>MSQFDILCKTPPKVLVRQFVERFERPSGEKIASCAAELTYLCWMITHNGTAIKRATFMSYNTIISNSLSFDIVNKSLQFKYKTQKATILEASLKKLIPAWEFTIIPYNGQKHQSDITDIVSSLQLQFESSEEADKGNSHSKKMLKALLSEGESIWEITEKILNSFEYTSRFTKTKTLYQFLFLATFINCGRFSDIKNVDPKSFKLVQNKYLGVIIQCLVTETKTSVSRHIYFFSARGRIDPLVYLDEFLRNSEPVLKRVNRTGNSSSNKQEYQLLKDNLVRSYNKALKKNAPYPIFAIKNGPKSHIGRHLMTSFLSMKGLTELTNVVGNWSDKRASAVARTTYTHQITAIPDHYFALVSRYYAYDPISKE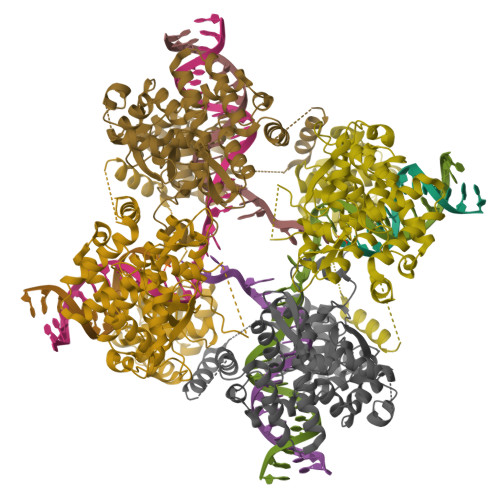MIALKDETNPIEEWQHIEQLKGSAEGSIRYPAWNGIISQEVLDYLSSYINRRI[4x]> GSEFQNKNFRAPQSEAIGILYKLIETGSKHKNMYDHTEITTDSLLALLGSEKVKIIDVRSADAYNGWRMRGEVRGGHIKGAKSLPAKWLTDPEWLNIVRFKQIRPEDAIVLYGYTPEECEQTATRFKENGYNNVSVFHRFHPDWTGNDAFPMDRLEQYNRLVPAEWVNGLISGEEIPEYDNDTFIVCHAHYRNRDAYLSGHIPGATDMDTLALESPETWNRRTPEELKKALEEHGITASTTVVLYGKFMHPDNADEFPGSAAGHIGAIRLAFIMMYAGVEDVRVLNGGYQSWTDAGFAISKDDVPKTTVPEFGAPIPSRPEFAVDIDEAKEMLQSEDSDLVCVRSYPEYIGEVSGYNYIKKKGRIPGAIFAECGSDAYHMENYRNHDHTTREYHEIEDIWAKSGIIPKKHL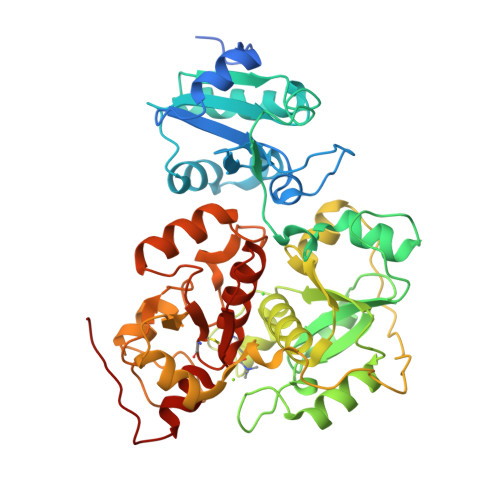AFYCGAGWRGSEAWFNALLMGWPRVSVYDGGWFEWSNDPENPYETGVPK In flies, Centrosomin (Cnn) forms a phosphorylation-dependent scaffold that recruits proteins to the mitotic centrosome, but how Cnn assembles into a scaffold is unclear. We show that scaffold assembly requires conserved leucine zipper (LZ) and Cnn-motif 2 (CM2) domains that co-assemble into a 2:2 complex in vitro. Purified CM2 forms a stable 2:2 tetramer with the purified LZ of the PReM domain, and we solve the crystal structure of the LZ:CM2 complex, revealing that helical dimers of LZ and CM2 interact in an anti-parallel fashion. Thus, Cnn molecules have an intrinsic ability to form large, LZ:CM2-interaction-dependent assemblies that are critical for mitotic centrosome assembly.

Most of these substitutions strongly perturbed the ability of the LZ to form a stable 2:2 tetramer with CM2, the only exception being L535E, which still formed a 2:2 tetramer but with reduced efficiency. Intriguingly, all of the individual LZ substitutions, including L535E, perturbed the assembly of the apo-LZ-homo-tetramer, and strongly reduced the α helicity of the proteins. To better understand why the L535E substitution did not more strongly disrupt the LZ:CM2 interaction, we generated LZ-L535E:CM2 crystals and solved their structure. Perhaps surprisingly, LZ-L535E appeared to be folded normally and was largely helical within the crystal structure. Although L535 is packed within the core of the LZ:CM2 assembly, there is sufficient space in the core to accommodate the longer E535 side chain, and E535 also forms a hydrogen bond with the invariant CM2 T1133 residue in the core. This presumably explains why the L535E mutation only relatively mildly perturbs LZ:CM2 assembly in vitro and Cnn scaffold assembly in vivo. Most strikingly, however, the L535E substitution could still form a detectable, although less robust, Cnn scaffold; this is in excellent agreement with our analysis of the behavior of the LZ-L535E:CM2 complex in vitro.

>GGSHDCAKVDLENAELRRKLIRTKRAFEDTYEKLRMANKAKAQVEKDIKNQILKTHNVLRNVRSNMENEL[2x];>[2x]GPMDQQNSAVIGQLRLELQQARTEVETADKWRLECIDVCSVLTNRLEEEAGFLNSLLK>AAPTAYTPLDVAQAYQFPEGLDGQGQCIAIIELGGGYDETSLAQYFASLGVSAPQVVSVSVDGATNQPTGDPNGPDGEVELDIEVAGALAPGAKIAVYFAPNTDAGFLNAITTAVHDPTHKPSIVSISW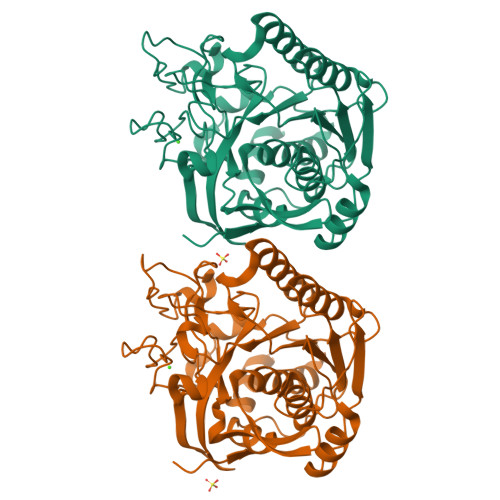GGPEDSWAPASIAAMNRAFLDAAALGVTVLAAAGDSGSTDGEQDGLYHVDFPAASPYVLACGGTRLVASAGRIERETVWNDGPDGGSTGGGVSRIFPLPSWQERANVPPSANPGAGSGRGVPDVAGNADPATGYEVVIDGETTVIGGTSAVAPLFAALVARINQKLGKPVGYLNPTLYQLPPEVFHDITEGNNDIANRARIYQAGPGWDPCTGLGSPIGIRLLQALLP[2x]>GAMATEQIQHIAIVGSVHGKYREMYRQLSEYEKSTGKEISFVICTGDMQTLRYEADLVYLKVPPKYKQMGDFHLYYEGKEKAPYLTLFIGGNHESSNVLLHLYNGGFVCFNMYYLGVCSCININGLRIVGVSGIYKSFDEKKPYTYPPSPNDVVSLFHTRNYVIQMLSNLSQSSQIDISLSHDWPQGIVMKGNYKQLYRFQPGFKKDGASLGSPINKVILNTLK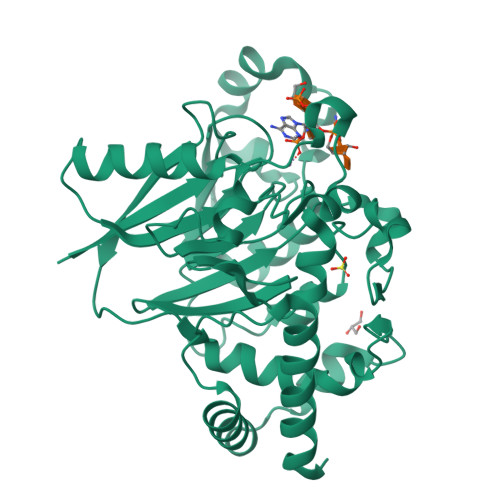PKYWISGHMHCEYHAEEGPTHFIALGKIGYKNAISYLDLPLKQKTDLEYDKDWVCNLIMTWPAFSNKAQFPDLSYSISELLSKRTKELDKKIIELWEKYIGLKIIYDSDTFDIQFTSRRFYIEKIYNELNIN[5x]Phosphoethanolamine (pEtN) cellulose is a naturally occurring modified cellulose produced by several Enterobacteriaceae. The minimal components of the E. coli cellulose synthase complex include the catalytically active BcsA enzyme, a hexameric semicircle of the periplasmic BcsB protein, and the outer membrane (OM)-integrated BcsC subunit containing periplasmic tetratricopeptide repeats (TPR). Additional subunits include BcsG, a membrane-anchored periplasmic pEtN transferase associated with BcsA, and BcsZ, a periplasmic cellulase of unknown biological function. Cellulose is a common bacterial biofilm component produced by a variety of prokaryotes, such as Escherichia coli (Ec), Salmonella enterica, and Gluconacetobacter/Komagataeibacter xylinus (Gx). These Gram-negative bacteria synthesize cellulose and secrete it across the cell envelope via the Bacterial cellulose synthase (Bcs) complex.

Although only the TM regions were resolved, the subunits were located ‘in front’ of BcsA near the periplasmic exit of its cellulose translocation channel. Taking advantage of recent improvements in 3-dimensional variability analyses and classifications implemented in the cryoSPARC data processing workflows, we reprocessed the previously published cryo-EM data (EMD-23267)20 focusing on the BcsA-BcsG complex, Fig. S2. Interprotomer contacts within the BcsG trimer are mediated by TM helix 4 of one subunit and TM helices 2 and 5 of a neighboring subunit, suggesting that BcsG is prone to self-polymerize. To test whether the NTD mediates interactions with BcsG, we performed AlphaFold2 complex predictions using either the full-length BcsA sequence or its NTD alone, together with three copies of BcsG’s TM region. The predictions reproducibly suggest the coordination of a BcsG trimer via BcsA’s NTD, Figs. 1f and S4b, which is predicted to fold into five short helices (α1-α5). The C-terminal helical region of Ec BcsA runs roughly in the opposite direction as the preceding amphipathic helix, which is present in BcsA from Rs and other species. This segment is resolved in our cryo-EM map and interacts with helix α5 of the NTD via an SxxPRxP motif (residues 850–856), Figs. 1e, f and S4a. No direct interactions are observed or predicted between BcsG and BcsA TM segments. The BcsG TM helices fit seamlessly into the opening of the BcsB semicircle, between the first and sixth subunit, Fig. 1e. Our cryo-EM analysis of the IM-associated Bcs complex reveals a single BcsA cellulose synthase associated with a trimer of the pEtN transferase BcsG.

>[6x]AWSHPQFEKTPATQPLINAEPAVAAQTEQNPQVGQVMPGVQGADAPVVAQNGPSRDVKLTFAQIAPPPGSMVLRGINPNGSIEFGMRSDEVVTKAMLNLEYTPSPSLLPVQSQLKVYLNDELMGVLPVTKEQLGKKTLAQMPINPLFISDFNRVRLEFVGHYQDVCEKPASTTLWLDVGRSSGLDLTYQTLNVKNDLSHFPVPFFDPSDNRTNTLPMVFAGAPDVGLQQASAIVASWFGSRSGWRGQNFPVLYNQLPDRNAIVFATNDKRPDFLRDHPAVKAPVIEMINHPQNPYVKLLVVFGRDDKDLLQAAKGIAQGNILFRGESVVVNEVKPLLPRKPYDAPNWVRTDRPVTFGELKTYEEQLQSSGLEPAAINVSLNLPPDLYLMRSTGIDMDINYRYTMPPVKDSSRMDISLNNQFLQSFNLSSKQEANRLLLRIPVLQGLLDGKTDVSIPALKLGATNQLRFDFEYMNPMPGGSVDNCITFQPVQNHVVIGDDSTIDFSKYYHFIPMPDLRAFANAGFPFSRMADLSQTITVMPKAPNEAQMETLLNTVGFIGAQTGFPAINLTVTDDGSTIQGKDADIMIIGGIPDKLKDDKQIDLLVQATESWVKTPMRQTPFPGIVPDESDRAAETRSTLTSSGAMAAVIGFQSPYNDQRSVIALLADSPRGYEMLNDAVNDSGKRATMFGSVAVIRESGINSLRVGDVYYVGHLPWFERVWYALANHPILLAVLAAISVILLAWVLWRLLRIISRRRLNPDNE;>MTQFTQNTAMPSSLWQYWRGLSGWNFYFLVKFGLLWAGYLNFHPLLNLVFAAFLLMPLPRYSLHRLRHWIALPIGFALFWHDTWLPGPESIMSQGSQVAGFSTDYLIDLVTRFINWQMIGAIFVLLVAWLFLSQWIRITVFVVAILLWLNVLTLAGPSFSLWPAGQPTTTVTTTGGNAAATVAATGGAPVVGDMPAQTAPPTTANLNAWLNNFYNAEAKRKSTFPSSLPADAQPFELLVINICSLSWSDIEAAGLMSHPLWSHFDIEFKNFNSATSYSGPAAIRLLRASCGQTSHTNLYQPANNDCYLFDNLSKLGFTQHLMMGHNGQFGGFLKEVRENGGMQSELMDQTNLPVILLGFDGSPVYDDTAVLNRWLDVTEKDKNSRSATFYNTLPLHDGNHYPGVSKTADYKARAQKFFDELDAFFTELEKSGRKVMVVVVPEHGGALKGDRMQVSGLRDIPSPSITDVPVGVKFFGMKAPHQGAPIVIEQPSSFLAISDLVVRVLDGKIFTEDNVDWKKLTSGLPQTAPVSENSNAVVIQYQDKPYVRLNGGDWVPYPQDYKDDDDK[3x];> MGSILTRWLLIPPVNARLIGRYRDYRRHGASAFSATLGCFWMILAWIFIPLEHPRWQRIRAEHKNLYPHINASRPRPLDPVRYLIQTCWLLIGASRKETPKPRRRAFSGLQNIRGRYHQWMNELPERVSHKTQHLDEKKELGHLSAGARRLILGIIVTFSLILALICVTQPFNPLAQFIFLMLLWGVALIVRRMPGRFSALMLIVLSLTVSCRYIWWRYTSTLNWDDPVSLVCGLILLFAETYAWIVLVLGYFQVVWPLNRQPVPLPKDMSLWPSVDIFVPTYNEDLNVVKNTIYASLGIDWPKDKLNIWILDDGGREEFRQFAQNVGVKYIARTTHEHAKAGNINNALKYAKGEFVSIFDCDHVPTRSFLQMTMGWFLKEKQLAMMQTPHHFFSPDPFERNLGRFRKTPNEGTLFYGLVQDGNDMWDATFFCGSCAVIRRKPLDEIGGIAVETVTEDAHTSLRLHRRGYTSAYMRIPQAAGLATESLSAHIGQRIRWARGMVQIFRLDNPLTGKGLKFAQRLCYVNAMFHFLSGIPRLIFLTAPLAFLLLHAYIIYAPALMIALFVLPHMIHASLTNSKIQGKYRHSFWSEIYETVLAWYIAPPTLVALINPHKGKFNVTAKGGLVEEEYVDWVISRPYIFLVLLNLVGVAVGIWRYFYGPPTEMLTVVVSMVWVFYNLIVLGGAVAVSVESKQVRRSHRVEMTMPAAIAREDGHLFSCTVQDFSDGGLGIKINGQAQILEGQKVNLLLKRGQQEYVFPTQVARVMGNEVGLKLMPLTTQQHIDFVQCTFARADTWALWQDSYPEDKPLESLLDILKLGFRGYRHLAEFAPSSVKGIFRVLTSLVSWVVSFIPRRPERSETAQPSDQALAQQHHHHHHLEHHHHHH> MHHHHHHKNIINTSILNLRYESNHLIDLSRYASEINIGSKVNFDPIDKNQIQLFNLESSKIEIILKNAIVYNSMYENFSTSFWIKIPKYFSKINLNNEYTIINCIENNSGWKVSLNYGEIIWTLQDNKQNIQRVVFKYSQMVAISDYINRWIFITITNNRLNNSKIYINGRLIDQKPISNLGNIHASNNIMFKLDGCRDPQRYIWIKYFNLFDKELNEKEIKDLYDNQSNSGILKDFWGNYLQYDKPYYMLNLYDPNKYVDVNNVGIRGYMYLKGPRGSIVTTNIYLNSSLYMGTKFIIKKYASGNKDNIVRNNDRVYINVVVKNKEYR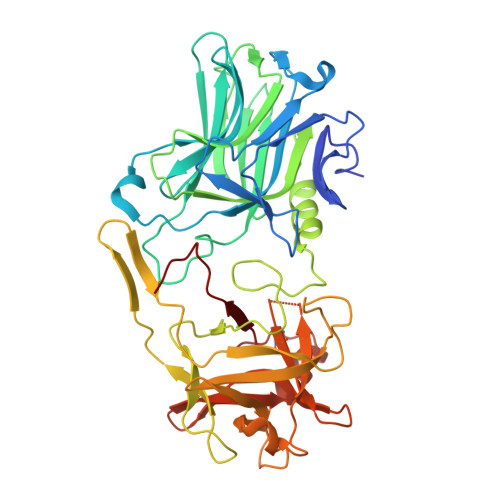LATNASQAGVEKILSVLEIPDVGNLSQVVVMKSKNDQGIRNKCKMNLQDNNGNDIGFIGFHQFNNIDKLVASNWYNRQIERSSRTFGCSWEFIPVDDGWGESPL>SNAADKVVQAGETVNDGTLTNHDNQIVFGTANGMTISTGLELGPDSEENTGGQWIQNGGIAGNTTVTTNGRQVVLEGGTASDTVIRDGGGQSLNGLAVNTTLNNRGEQWVHEGGVATGTIINRDGYQSVKSGGLATGTIINTGAEGGPDSDNSYTGQKVQGTAESTTINKNGRQIILFSGLARDTLIYAGGDQSVHGRALNTTLNGGYQYVHRDGLALNTVINEGGWQVVKAGGAAGNTTINQNGELRVHAGGEATAVTQNTGGALVTSTAATVIGTNRLGNFTVENGKADGVVLESGGRLDVLESHSAQNTLVDDGGTLAVSAGGKATSVTITSGGALIADSGATVEGTNASGKFSIDGTSGQASGLLLENGGSFTVNAGGQAGNTTVGHRGTLTLAAGGSLSGRTQLSKGASMVLNGDVVS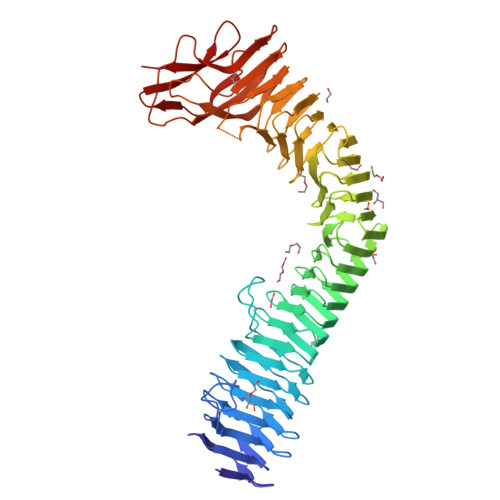TGDIVNAGEIRFDNQTTPNAALSRAVAKSNSPVTFHKLTTTNLTGQGGTINMRVRLDGSNASDQLVINGGQATGKTWLAFTNVGNSNLGVATTGQGIRVVDAQNGATTEEGAFALSRPLQAGAFNYTLNRDSDEDWYLRSEN[4x]> GMANDQDLSNPEYLYTEDDINQLLKHYLGLDDRISIIQHVALNESLLLKQTLHQVLSDIFSGMQEKAVIPLHTGNNHWVAMAIKKGMNDDIVISYNDPMGVSIDDKVTLINCIKELCPGAKINDLQTVQQTNVYDCGPFVVDNLIKMSQGQPILSTEEAKQQAQNIRQSQVNFLSENRMITSAAAALADTLLKNNNRITEGVLVDRIFDNKILSVQEKQQLLNNLLDNHIKENKSLTKESLTRMLASTHFVQQQANVLLN

Here we report biochemical and structural data on the DUB domain of O. tsutsugamushi OTT_1962, hereafter called OtDUB. Primary sequence analysis revealed conservation of a DUB-like catalytic triad (His76, Asp96, Cys135) and Trp77, suggesting that the Ulp1-like domain is catalytically active and not an acetyltransferase, respectively. OtDUB preferentially cleaves ubiquitin chains having at least three ubiquitins and efficiently cleaves both K48- and K63-linked chains, unlike other members of this clan that prefer K63 chains. In summary, we have uncovered a unique DUB from the obligate intracellular pathogen O. tsutsugamushi that is capable of efficiently cleaving long ubiquitin chains of different linkages and binding ubiquitin with extraordinary affinity.

We cloned the N-terminal domain of OtDUB from genomic DNA of the O. tsutsugamushi Ikeda isolate and included residues past the putative DUB domain (1–311) to examine a potential accessory domain that could modulate DUB activity. We determined the crystal structure of the apo-enzyme at 2.0 Å resolution, which revealed that the Ulp1-like domain of OtDUB has the predicted core fold of cysteine endopeptidase (CE)-clan proteases. OtDUB lacks an N-terminal VR-1; instead, the C-terminal accessory domain (residues 170–259) protrudes into the VR-1 position via an extended α-helical arm positioned close to the catalytic site, suggesting that it assists in substrate binding. The C-terminal region of the protein fragment, residues 260–311, was apparently disordered and not observed in the structure. When compared to the phylogenetically closest structure, RickCE from Rickettsia bellii, we observed structural conservation of only one VR: the small loop in VR-3. Besides lacking the N-terminal VR-1 present in RickCE, VR-2 of OtDUB comprises a loop and two short α-helices, while RickCE VR-2 is a large helical arm largely absent in OtDUB. These large structural differences between the two DUBs, and other prokaryotic CE-clan structures, are obvious when aligned, yet the core protease fold is conserved (Cα root-mean-square deviation (RMSD) 1.2–3.9 Å). A substantial structural transition of the UBD was supported by the apo-DUB-UBD1–311 crystal structure, which lacked density for residues 224–235 at the beginning of the UBD, a region that includes the ubiquitin-interacting residues D226 and K230.> MTAAVTPSASAVASDDKKSERRLAFWLIAPAVLLMLAVTAYPIGYAVWLSLQRYNLAEPHDTEFIGLANYVTVLTDGYWWTAFAVTLGITVVSVAIEFALGLALALVMHRTIFGKGAVRTAILIPYGIVTVAASYSWYYAWTPGTGYLANLLPEGSAPLTDQLPSLAIVVLAEVWKTTPFMALLLLAGLALVPQDLLNAAQVDGAGPWKRLTKVILPMIKPAILVALLFRTLDAFRIFDNIYILTGGSNDTGSVSILGYDNLFKAFNVGLGSAISVLIFLSVAIIAFIYIKIFGAAAPGSDEEVR;> MADRVDARRATWWSVVNILVIVYALIPVLWILSLSLKPTSSVKDGKLIPTEITFANYKAIFSGDAFTSALFNSIGIGLITTIIAVVIGGMAAYAVARLQFPGKQLLIGVALLIAMFPHISLVTPIFNMWRGIGLFDTWPGLIIPYITFALPLAIYTLSAFFREIPWDLEKAAKMDGATPAQAFRKVIAPLAAPGIVTAAILVFIFAWNDLLLALSLTATQRAITAPVAIANFTGSSQFEEPTGSIAAGAMVITIPIIIFVLIFQRRIVAGLTS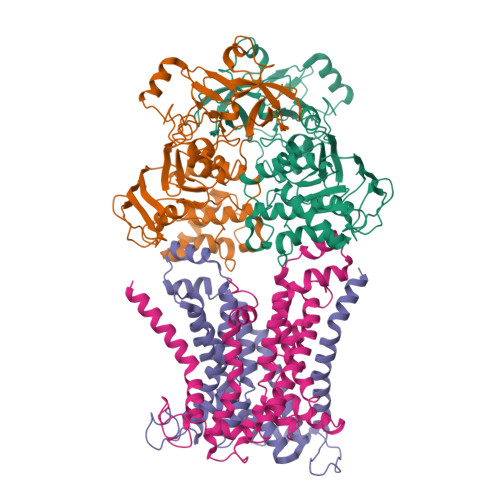GAVKG;>MAEIVLDRVTKSYPDGAGGVRAAVKEFSMTIADGEFIILVGPSGCGKSTTLNMIAGLEEITSGELRIGGERVNEKAPKDRDIAMVFQSYALYPHMTVRQNIAFPLTLAKVPKAEIAAKVEETAKILDLSELLDRKPGQLSGGQRQRVAMGRAIVRSPKAFLMDEPLSNLDAKLRVQMRAEISRLQDRLGTTTVYVTHDQTEAMTLGDRVVVMLAGEVQQIGTPDELYSSPANLFVAGFIGSPAMNFFPATRTDVGVRLPFGEVTLTPHMLDLLDKQARPENIIVGIRPEHIEDSALLDGYARIRALTFSVRADIVESLGADKYVHFTTEGAGAESAQLAELAADSGAGTNQFIARVSADSRVRTGEQIELAIDTTKLSIFDAATGLNLTRDITPTDPTEAAGPDAG[2x]> 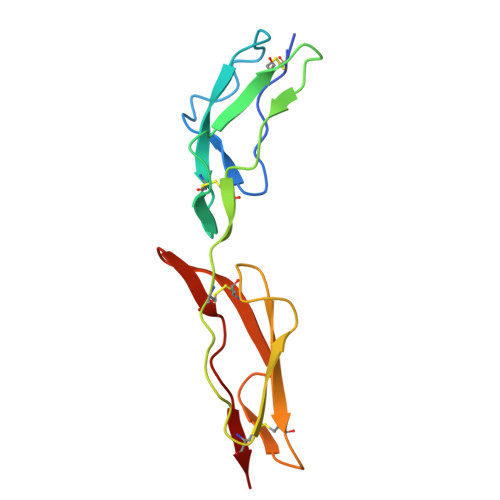GPGSNCGPPPTLSFAAPMDITLTETRFKTGTTLKYTCLPGYVRSHSTQTLTCNSDGEWVYNTFCIYKRCRHPGELRNGQVEIKTDLSFGSQIEFSCSEGFFLIGSTTSRCEVQDRGVGWSHPLPQCEI> ADPTEPSSPPGAPSQPVVTEITKNSITLTWKPNPQTGAAVTSYVI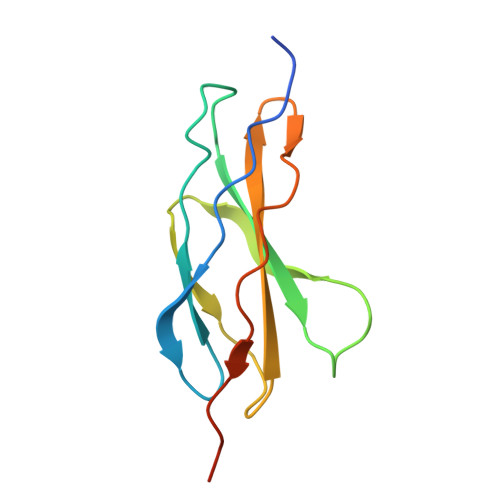EAFSPAAGNTWRTVADGVQLETHTVSGLQPNTIYLFLVRAVGAWGLSEPSPVSEPVRTQDSEFHHHHHH> MKKKMSKLNARVHDFSMFKGNHIPRSKIHIPHKTIRAFNVGEIIPIYQTPVYPGEHIKMDLTSLYRPSTFIVPPMDDLIVDTYAFAVPWRIVWKDLEKFFGENSDSWDVKNAPPVPDIVAPSGGWDYGTLADHFGITPKVPGIRVKSLRFRAYAKII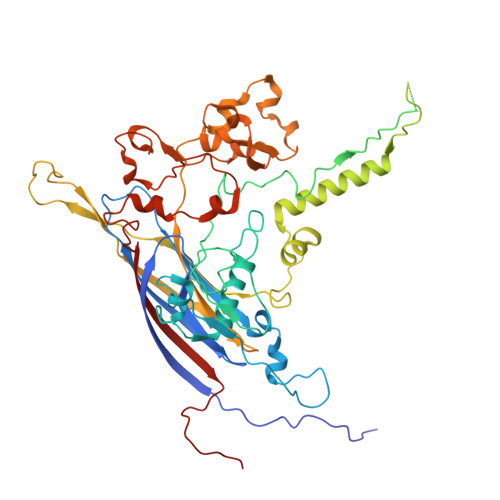NDWFRDQNLSSECALTLDSSNSQGSNGSNQVTDIQLGGKPYIANKYHDYFTSCLPAPQKGAPTTLNVGGMAPVTTKFRDVPNLSGTPLIFRDNKGRTIKTGQLGIGPVDAGFLVAQNTAQAANGERAIPSNLWADLSNATGISISDLRLAITYQHYKEMDARGGTRYVEFTLNHFGVHTADARLQRSEFLGGHSQSLLVQSVPQTSSTVEKMTPQGNLAAFSETMIQNNYLVNKTFTEHSYIIVLAVVRYKHTYQQGIEADWFRGQDKFDMYDPLLANISEQPVKNREIMVQGNSQDNEIFGFQEAWADLRFKPNSVAGVMRSSHPQSLDYWHFADHYAQLPKLSSEWLKEDYKNVDRTLALKASDNTPQLRVDFMFNTIAEKPMPLYSTPGLRRI N-({(3S,4S)-4-[(benzylsulfonyl)amino]pyrrolidin-3-yl}methyl)-4-methoxy-3-(3-methoxypropoxy)-N-(propan-2-yl)benzamide | C27 H39 N3 O6 S | 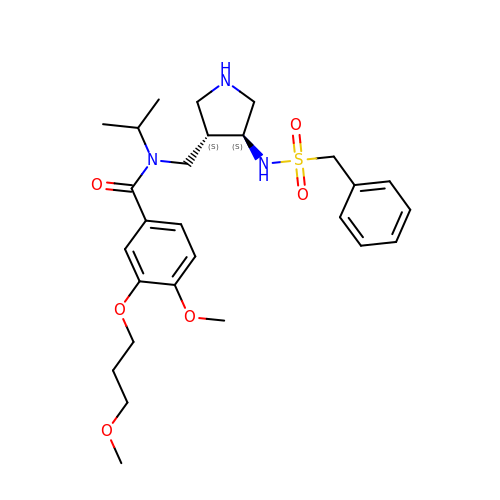WPSURGXSNWIBBJ-BJKOFHAPSA-N> DPSKDSKAQVSAAEAGITGTWYNQLGSTFIVTAGADGALTGTYESAVGNAESRYVLTGRYDS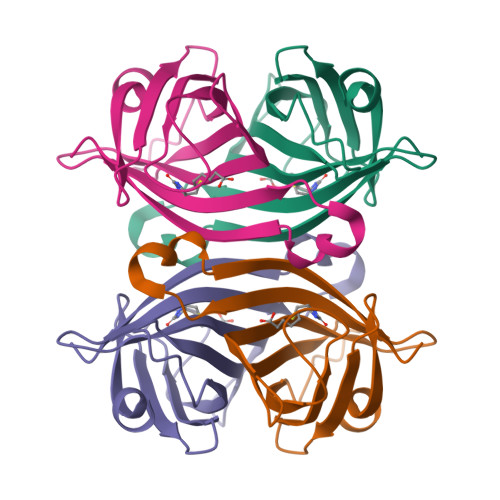APATDGSGTALGWTVAWKNNYRNAHSATTWSGQYVGGAEARINTQWLLTSGTTEANAWKSTLVGHDTFTKVKPSAASIDAAKKAGVNNGNPLDAVQQ Autophagy-related protein 18 (Atg18) participates in the elongation of early autophagosomal structures in concert with Atg2 and Atg9 complexes. Atg18 belongs to the protein family of β-propellers that bind polyphosphoinositides (PROPPIN). The corresponding primary structure contains a series of conserved WD40 repeats forming the 6 or 7 blades of a β-propeller fold. The autophagic membrane adapter Atg18 reveals an unexpected structural plasticity in multiple modes of oligomeric organization.

To further investigate the binding mode of Atg18 to lipid membranes, we mixed soluble Atg18 with PI3,5P2-doped large unilamellar vesicles (LUVs). The membrane surfaces are typically coated by disc-shaped particles corresponding to Atg18 β-propellers in dimension. When membranes are aligned in parallel, we found connecting density that we interpreted as Atg18 bridging two juxtaposed bilayers. The inter-membrane distance in the Atg18-WT and Atg18 s-loop samples was constant over parallel membrane stretches and very similar at ~80 Å, respectively, whereas no consistent inter-membrane spacing could be detected between undecorated 100% DOPC liposomes without Atg18. Further 3D subclassification resulted in a structure of two S-shaped densities packed against each other made up of eight disc-shaped densities with ~50 Å diameter each. In the density, we found Atg18 molecules in four pairs of dimers with a slightly twisted interface matching the observed I-interface of the tubular Atg18 assembly determined above. Notably in the cryo-EM density, the basic Atg18 dimer unit was found to assume a 45° tilt angle with respect to both membrane planes, which could be independently confirmed by measurements in raw tomogram slices. The rigid body fit of the Atg18 dimer was consistent with the location of the PI3P binding sites as well as the 6CD loop facing opposing membrane bilayers. The fitted Atg18 dimers lack the interaction through the T-interface due to PIP-binding.

>[8x]MSDSSPTINFINFNQTGTCISLGTSKGFKIFNCEPFGKFYSEDSGGYAIVEMLFSTSLLALVGIGDQPALSAARLRIINTKKHSIICEVTFPTSILSVKMNKSRLVVLLQEQIYIYDINTMRLLHTIETNPNPRGLMAMSPSVANSYLVYPSPPKVINSEIKAHATTNNITLSVGGNTETSFKRDQQDAGHSDISDLDQYSSFTKRDDADPTSSNGGNSSIIKNGDVIVFNLETLQPTMVIEAHKGEIAAMAISFDGTLMATASDKGTIIRVFDIETGDKIYQFRRGTYATRIYSISFSEDSQYLAVTGSSKTVHIFKLGHSMSNNKLDSDDSNMEEAAADDSSLDTTSIDALSDEENPTRLAREPYVDASRKTMGRMIRYSSQKLSRRAARTLGQIFPIKVTSLLESSRHFASLKLPVETNSHVMTISSIGSPIDIDTSEYPELFETGNSASTESYHEPVMKMVPIRVVSSDGYLYNFVMDPERGGDCLILSQYSILMD> MGSSHHHHHHSSGENLYFQG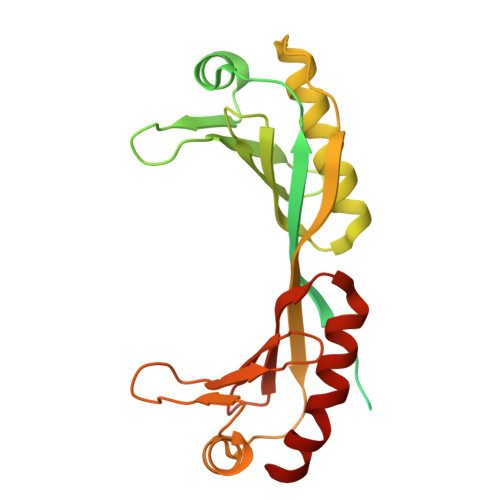HMEAIQTHPANAAQAKAFTAPGSLSFPGGASEIANSTAPTNGASNGGQQQGVQATSGAGVTPATPAATPGAGPAGPSGITPTLQNIVATVNLDCRLDLKTIALHARNAEYNPKRFAAVIMRIREPKTTALIFASGKMVVTGAKSEDDSKLASRKYARIIQKLGFNAKFTDFKIQNIVGSCDIKFPIRLEGLASKHHNFSSYEPELFPGLIYRMIKPKIVLLIFVSGKIVLTGAKVREEIYQAFEMIYPVLQDFRKV>[2x]GAMAQHEVITRGGDAFLLKLRESALSSGSMSEEQFFLLIGISSIHSDRV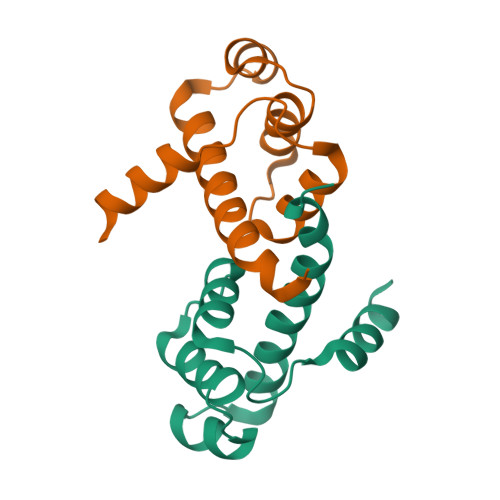ILAMKDYLVSGHSRKDVCEKYQMNNGYFSTTLGRLTRLNVLVARLAPYYTDSVSAIAEAASL> SALTPQLKDTLEKLVNSEKVVLFMKGTRDFPMCGFSNTVVQILK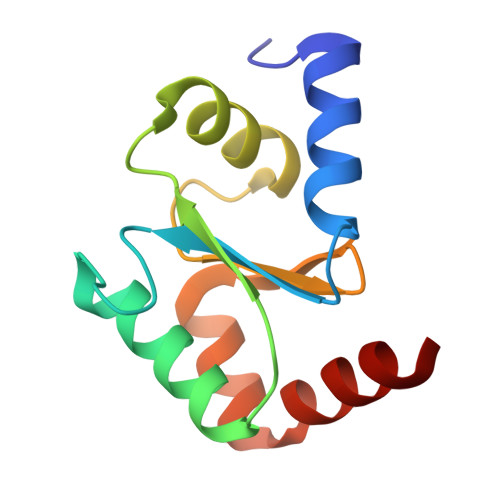NLNVPFEDVNILENEMLRQGLKEYSNWPTFPQLYIGGEFFGGCDITLEAFKTGELQEEVEKAMCS>DAAPAAGSTLDKIAKNGVIVVGHRESSVPFSYYDNQQKVVGYSQDYSNAIVEAVKKKLNKPDLQVKLIPITSQNRIPLLQNGTFDFECGSTTNNVERQKQAAFSDTIFVVGTRLLTKKGGDIKDFADLKGKAVVVTSGTTSEVLLNKLNEEQKMNMRIISAKDHGDSFRTLESGRAVAFMMDDALLAGERAKAKKPDNWDIVGKPQSQEAYGCMLRKDDPQFKKLMDDTIAQVQTSGEAEKWFDKWFKNP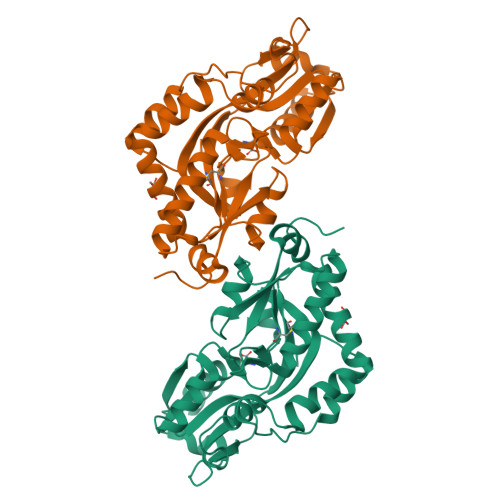IPPKNLNMNFELSDEMKALFKEPNDKALNLEHHHHHH[2x]M. smegmatis Nei2, so named by virtue of its homology to Escherichia coli endonuclease VIII (Nei), is a 252-aa monomeric enzyme with AP β-lyase activity on single-stranded DNA. The lhr–nei2 gene operon of Mycobacterium tuberculosis and its avirulent relative Mycobacterium smegmatis encodes a pair of enzymes implicated in DNA repair: the Lhr helicase and the Nei2 AP lyase (1–4). Expression of Nei2, and its operonic neighbor Lhr (a tetrameric 3′-to-5′ helicase), is induced in mycobacteria exposed to DNA damaging agents. We demonstrate here that Nei2 has 5-hydroxyuracil glycosylase/β-lyase activity on single-stranded DNA.

Here, we crystalized Nei2 and determined its structure at 1.45 Å resolution. The refined Nei2 model (Rwork/Rfree = 16.7/20.5) comprised a continuous polypeptide from Pro2 to Ala251. There was no density for the N-terminal methionine, which we presume was removed by methionine aminopeptidase during Nei2 expression in E. coli. The protein consists of an N-terminal lobe (aa 2–116) and a C-terminal lobe (aa 123–251) connected by a linker peptide. The N lobe is built around two four-strand antiparallel β-sheets (β1↑•β6↓•β7↑•β5↓ and β2↑•β3↓•β4↑•β8↓) that form a β-sandwich, which is flanked by the N-terminal α1 helix and two short 310 helices. The C domain comprises a 4-helix bundle, a β9-β10 hairpin, and a tetracysteine-zinc complex. A strong anomalous difference peak was detected overlying the modeled zinc atom. Weaker anomalous peaks were detected over the Sγ atoms of Cys225, Cys228, Cys245, and Cys248 that bind the zinc ion. The N and C lobes are arranged in a saddle-like shape with a deep groove between them, in which the N-terminal proline (Pro2) is located, thereby demarcating the AP lyase active site. The saddle groove is lined by positive electrostatic potential that provides a docking site for the DNA substrate, as seen in structures of AP lyase-related enzymes.

> MPEGDTVFHTAAALRAALEGKTLTRCDVRVPRYATVDLSGAVVDEVLSRGKHLFIRAGSASIHSHLKMEGAWRIGHTKVAPHRIRIVLETADTRAIGIDLGILEVLDRGTDMDAVAYLGPDLLGPDWEPRVAADNLAADPDRPLAQALLDQRVMAGVGNVYCNELCFVFGRLPTAPVGTLKDPLRVVQRARDMLWLNRSRWNRTTTGDTRNGRQLWVYGRAGEPCRRCGTLIQTDRGGERVTYWCPVCQTASLEHHHHHH> MAEYQDKVVDVEVSLGTQPIDTVGFETPMFLAMHGNFPERIRFYVSTAGMVADGFAVGSPAYQFATNAFAGNFAPQRVAIGRMSIDSSKVDFTGTTNTEQVVVNITLNKVVKAVKINVLPGNTPAQIATALADAVTADADLTGKATAVATGTYVTVTAVSPNVVSVGKGAGVYKIVNESSETVATVLPSVIAENHNWYFLATEARSDADIVAAAEFAKANYKLHIYNSTDVDAYAPENSAASVFDTLKSLSYDSLGTSDAGADVDFTEGSVIGAMAANDPSYGDSLHLKTMPGMVPFAGSDTQRSNAWSRNANIYRGLYGGGSYIEGKTSSGQYVDVIRFSHWVKFRMEESVFAYMKRRSDMGLSMKMSDEDLPVLKSVLMNNPINIGIRNGGILTGYDTENKVSYDPTIIIPKRANIPTNDLAARILRDVKVELVYNNSLHYVKIRASVVLDRPAGQSTNAQTPMSSSAVGV;> MLNQSKILTLQAYD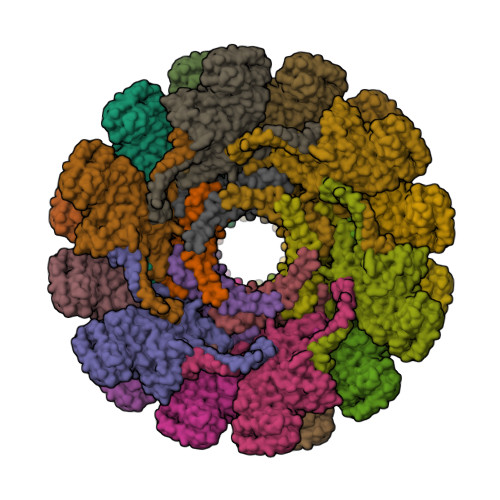PAKVLVFIGGQRVSGFAADTKIVITRNNDNISVHAGVDGEISNALSRDNTGVMTLSLQNTAKWNGYLAQWQRQANVTGLIYLPVQVEGSQGLSLNTIGWIQKQPDLSYGTEVGQMDWEIGVLDAWLSPDQIQGIAAGITGLLGLDQ>[6x]MHLPNGAQIFVETSRGVEVEATAITNAENPVATVASKGDLAKGDYVIVTQSTWAKMVSRVLIVTDAQETSITLAGIDTSDTLVFPAGGTMSFAKITGWTEIPCVQEIGQDGGEQQYYTYQCLSDDKEQQIPTFKSAVSLTYTFAHEFDNPIYPILRKLDSSGQVTAVRMYVPKASEMRMWAGILSFNDIPSTQVNEMETVELAVSLKGDFTFISSTLASPGA

Siphophage T1 is representative of the T series of model Escherichia coli phages, which has been observed to infect not only sensitive strains of E. coli but also some strains of Shigella dysenteriae. Siphophages possess a long, flexible, and non-contractile tail that plays a crucial role in host recognition, cell envelope penetration, and DNA injection. Connected to the head through a connector complex, the tail of a siphophage consists of three main components: a tail tube, a tape measure protein (TMP), and a distal tip. Using cryo-EM, we resolved the three-dimensional (3D) structures of the icosahedral head, head–tail complex and the tail tip of a laboratory-adapted fiberless mature T1 at resolutions of 3.5 Å, 3.6 Å, and 4.3 Å, respectively.

The flexible tail tube comprises approximately 34 hexameric rings of tail tube. The extensive disulfide bond network along the successive tail rings may mediate the flexible bending. Notably, the flexible tail tube of T1 may be mediated by the disulfide bonds between two adjacent tail rings, which allows for more efficient capture of host receptors. Notably, besides the interspace and distance between successive rings and the β-hairpin domain that contribute to the tail flexibility of siphophages, the disulfide bond network along the entire tail tube may also mediate the flexibility of the T1 tail. The flexibility of the tail may enable the receptor-binding protein to explore larger spaces for the host receptor, resulting in enhancing their competition and adaptation to hostile environments.3,4-dihydro[1,2,4]triazolo[1,5-a][3,1]benzimidazol-9-ium | C8 H7 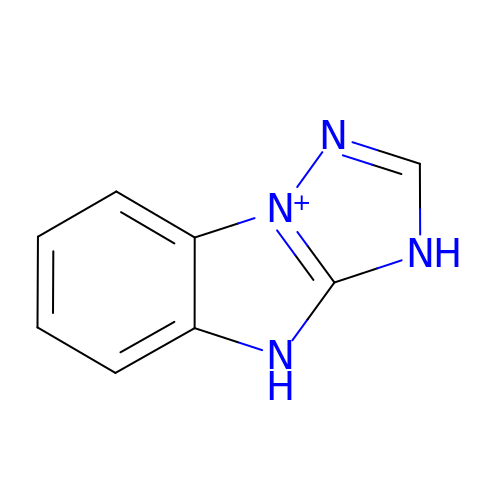N4 | UHMYOSZMUIJCFW-UHFFFAOYSA-O(3R,4S)-1-[(4-amino-5H-pyrrolo[3,2-d]pyrimidin-7-yl)methyl]-4-{[(prop-2-yn-1-yl)sulfanyl]methyl}pyrrolidin-3-ol | C15 H19 N5 O S | 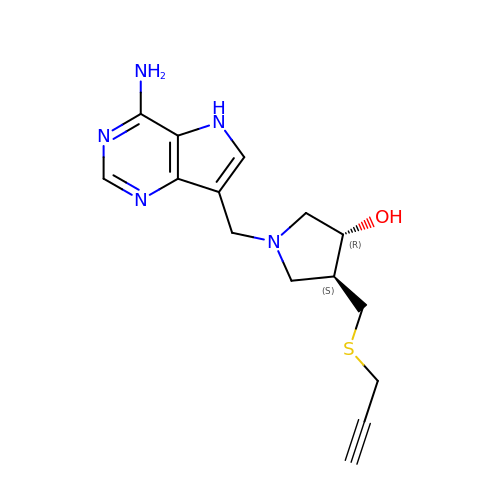MQJBNGGMAUMWEV-NEPJUHHUSA-N(R)-N-((1-(6-(benzylamino)pyrimidin-4-yl)-3-hydroxypiperidin-3-yl)methyl)-4-((4,4-dimethylpiperidin-1-yl)methyl)benzamide | C32 H42 N6 O2 | 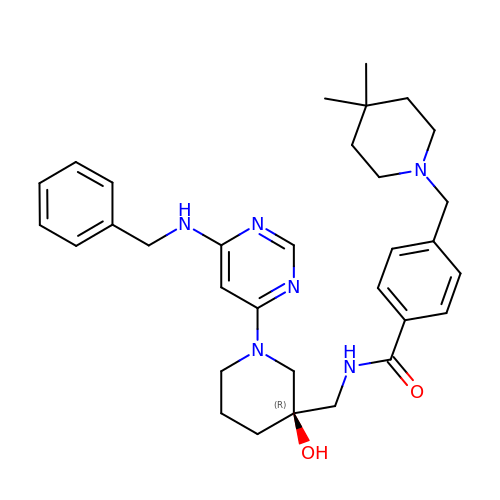UMNYWWVELYOOIU-JGCGQSQUSA-N> MKIGIIGAGQLARMLSLAGTPLGLEFHCLGKNGDCAEEVVKTVTDIELTKVNDVVAWAKQFDVITFENENISHELIKAINHEVSVYPSAKAIAISQDRLLEKSFMQDHGIATAKFVNIDSLAKLQSAVDDHGLPAILKTRRFGYDGKGQFVIRSQEDITKAWDVLKDAPDGLIYEAFVDFDYEVSQICTADLKGNIAFYPLARNTHKQG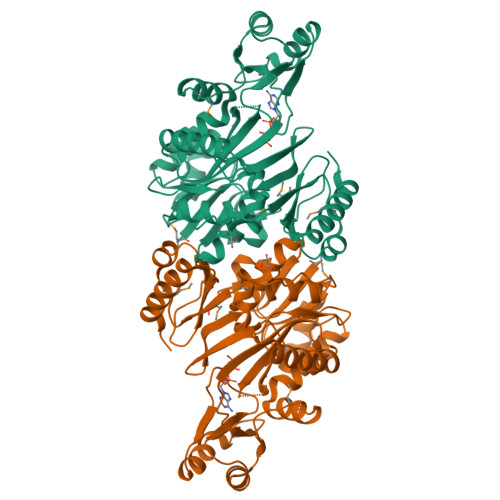IIVESEAPFENVVLAEKAQQIAKILVKEFAYVGTLAIEFFVKGDELIVNEIAPRVHNSGHWSIDGAVTSQFENHVRAIAGLILGDTTSRKTVMLNCIGGMPATKDLAALDRVKIHSYNKEPRKGRKVGHLNLNLNDETDEYQLLQVKKLIALSEEI>MKYILVTGGVISGVGKGVIASSFGTLLKSCGLDVTSIKIDPYINIDAGTFSPYEHGEVYVLDDGAEVDLDLGNYERFLDVTLHRDNNITTGKIYKLVIEKERTGEYLGKTVQVVPHITDAIQEWVERVAQTPVQGSSKPQVCIVELGGTIGDIEGMPFVEAFRQFQFRVKRENFCLAHVSLVPLPKATGEPKTKPTQSSVRELRGCGLSPDLIVCRSEKPIGLEVKEKISNFCHVGPDQVICIHDLNSIYHVPLLMEQNGVIEYLNERLQLNIDMSKRTKCLQQWRDLARRTETVRREVCIAVVGKYTKFTDSYASVVKALQHAALAVNRKLELVFIESCLLEEETLHSEPSKYHKEWQKLCDSHGILVPGGFGSRGMEGKIRACQWARENQKPLLGICLGLQAAVIEFARNKLGLKDANTTEIDPNTANALVIDMPEHHTGQLGGTMRLGKRITVFSDGPSVIRQLYGNPKSVQERHRHRYEVNPKYVHLLEEQGMRFVGTDVDKTRMEIIELSGHPYFVATQYHPEYLS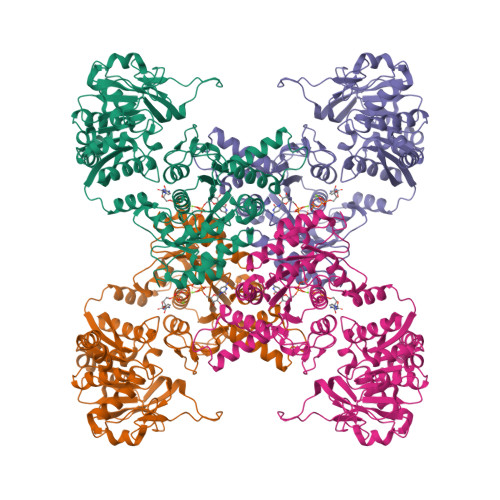RPLKPSPPFLGLILASVDRLNQYIQ[4x]> GSSHHHHHHHHHHSSGLVPRGSHMGDGYYKLVARHSGKALDVENASTSDGANVIQYSYSGGDNQQWRLVDLGDGYY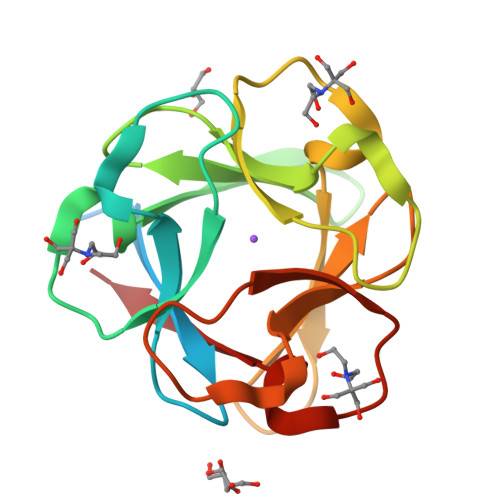KLVARHSGKALDVENASTSDGANVIQYSYSGGDNQQWRLVDLGDGYYKLVARHSGKALDVENASTSDGANVIQYSYSGGDNQQWRLVDL(2S)-2-HYDROXYPENTANEDIOIC ACID 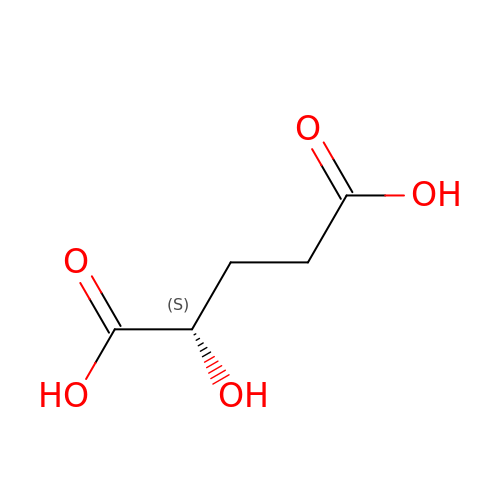| C5 H8 O5 | HWXBTNAVRSUOJR-VKHMYHEASA-N> MSRNDKEPFFVKFLKSSDNSKCFFKALESIKEFQSEEYLQIITEE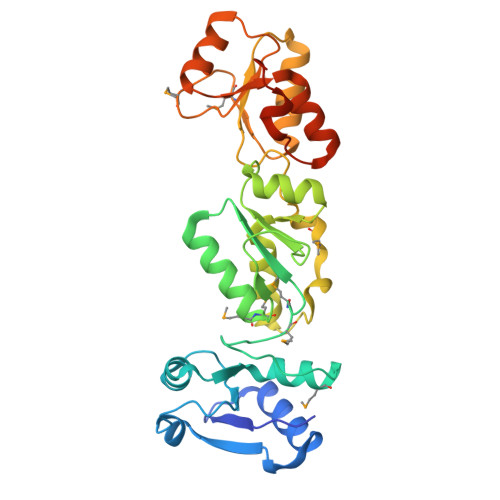EALKIKENDRSLYICDPFSGVVFDHLKKLGCRIVGPQVVIFCMHHQRCVPRAEHPVYNMVMSDVTISCTSLEKEKREEVHKYVQMMGGRVYRDLNVSVTHLIAGEVGSKKYLVAANLKKPILLPSWIKTLWEKSQEKKITRYTDINMEDFKCPIFLGCIICVTGLCGLDRKEVQQLTVKHGGQYMGQLKMNECTHLIVQEPKGQKYECAKRWNVHCVTTQWFFDSIEKGFCQDESIYKTEPRPEALEHHHHHH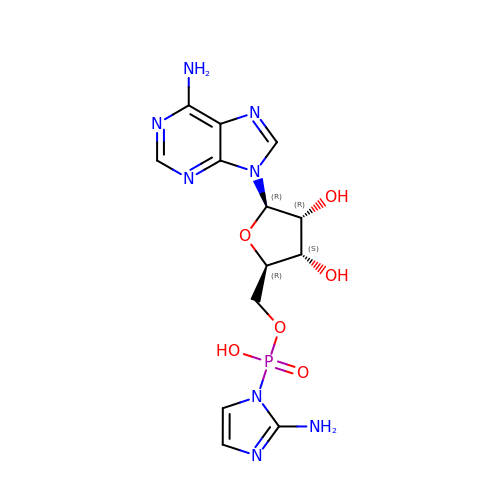5'-O-[(S)-(2-amino-1H-imidazol-1-yl)(hydroxy)phosphoryl]adenosine | C13 H17 N8 O6 P | VRUNWCWGNRYOCC-WOUKDFQISA-N> MKKTFNLVATAAAGIEAVVGKELRNLGLDCQVENGRVLFKGNIETIAKSNLWLRSADRIKIVVGEFPARTFEELFQGVYALDWENYLPLGCQFPVAKAKSVKSKLHNEPSIQGITKKAIVKKLQHYFHRPDSV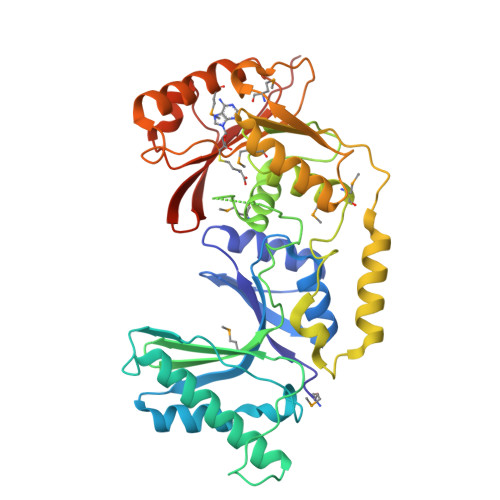PLPENGPEFKIEISLLKDQARVMIDTTGPSLFKRGYRTEKGGAPIKENMAAAIILLSNWFPDKPFVDPTCGSGTFCIEAAMIGMNIAPGFNRDFAFEEWPWVDEALVTRVRNEADEQADYDIQLDISGFDFDGRMVEIARKNAREVGLEDVVKLKQMRLQDFKTNKINGVLISNPPYGERLLDDKAVDILYNEMGETFAPLKTWSQFILTNDTDFEQKFGRKADKKRKLYNGSLKVDLYQFYGQRVKRVLR>GAMAKLMFDSILVICTGNICRSPIGERLLRRLLPSKKINSAGVGALVDHTADESAIRVAEKNGLCLKGHRGTKFTSALARQYDLLLV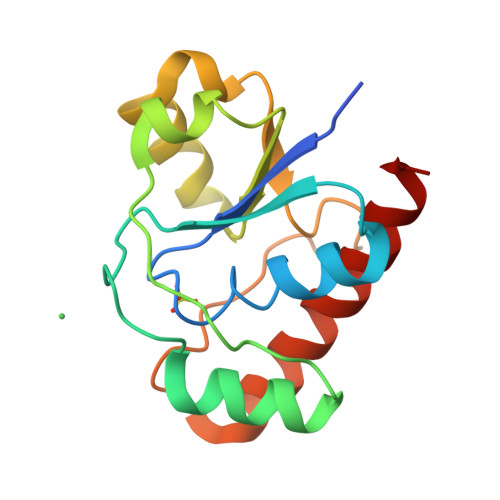MEYSHLEQISRIAPEARGKTMLFGHWLDSKEIPDPYRMSDEAFDSVYQLLEQASKRWAEKLGE[8x]> GSHKFAEKVEEIVAKNARAEIDYSDAPDEF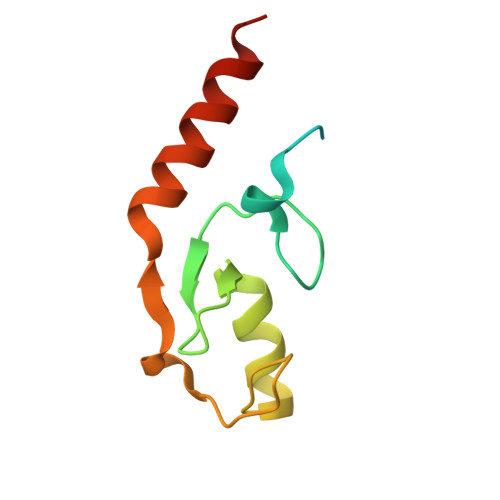RDPLMDTLMTDPVRLPSGTIMDRSIILRHLLNSPTDPFNRQTLTESMLEPVPELKEQIQAWMREKQNSDH> MSGKANASKKNAQQLKRNPKRKKDNEEVVLSENKVRNTVKKNKNHLKDLSSEGQTKHTNLKHGKTAASKRKTWQPLSKSTRDHLQTMMESVIMTI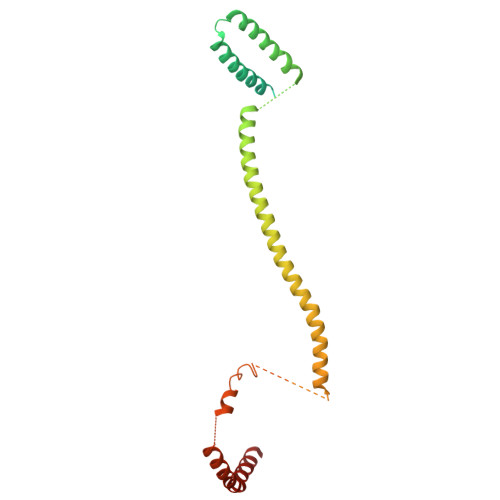LSNSIKEKEEIQYHLNFLKKRLLQQCETLKVPPKKMEDLTNVSSLLNMERARDKANEEGLALLQEEIDKMVETTELMTGNIQSLKNKIQILASEVEEEEERVKQMHQINSSGVLSLPELSQKTLKAPTLQKEILALIPNQNALLKDLDILHNSSQMKSMSTFIEEAYKKLDAS> MTRIVWMIGGAQGLGVDTSANIFGNAVAKAGYYLFGNREYYSNIKGRHSYFEVVISEKPIRSLSSYVNILASFDAETVFQHFTETKEYLIYNVEYENTTVDLVKSMEPEMAEQVKEALSKERLGFTIKDVLEYLKRRGVKVIGFNYTELIKKIADTFKVPMSVVERAKNMIAVGASYGLLGLKFDYLKDAISSTFKNELFIKFNTMAAELGYNSVPNVYKLQEYKIEKQRIQVDGNTISAMGKLAGGLRFQSYYPITPASDESVYIEANQNLDMIVEGNELRKGGVVVVQAEDELAAINMAVGAALTGVRSATATSGPGFSLMSEGISWAGMNEVPVVITYYMRGAPATGLPTRSGQADLKFALNVGHGEFPRIVIASGDHVEIFWDAIWALNLAEKYQTPVIHIIEKTLANAYSVFEEELITNRPYVIERGK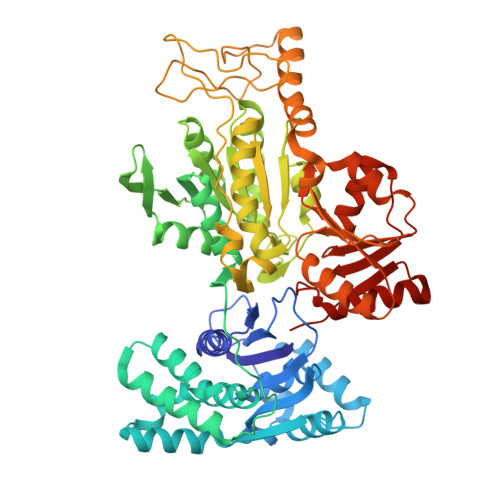IVKPTSDYFNRFEVTEDGISPRVFLGQASIFYTGDEHNEEGHITENSINRMKMYEKRNKKLETADKEIPEEQRVNIVGDADIVLLTWGSPKGAILDAMEELSKDGIKTMMVQVKMFNPYPKNLMKKILSGKSKIIAVENNYNAQGAEVLAEKTGIFATNYILKWTGRPITREEVIEGIKKILERDEKRVVLYGGA> GDQLTHVVEEVKTYDLVWRSIKNLWEDVQRTFETPWCRVDVLLLQSDLANFLRRADELPRAVKQFEMYKSLFSQVNMLTSVNKILVELKDGALKPRHWNMIFRDIGKRQIQKNLLDKLEFSLKDVMVLNLTLNEILLTKIIERAQKEFVIEKSLNRIKKFWKEAQYEVIEHSSGLKLVREWDVLEQACKEDLEELVSMKASNYYKIFEQDCLDLESKLTKLSEIQVNWVEVQFYWLDLYGILGENLDIQNFLPLETSKFKSLTSEYKMITTRAFQLDTTIEVIHIPNFDTTLKLTIDSLKMIKSSLSTFLERQRRQFPRFYFLGNDDLLKIIGSGKHHDQVSKFMKKMFGSIESIIFFEDSITGVRSVEGEVLNLNEKIELKDSIQAQEWLNILDTEIKLSVFTQFRDCLGQLKDGTDIEVVVSKYIFQAILLSAQVMWTELVEKCLQTNEFSKYWKEVDMKIKGLLDKLNKSSDNVKKKIEALLVEYLHFNNVIGQLKNCSTKEEARLLWAKVQKFYQKNDTLDDLNSVFISQSGYLLQYKFEYIGIPERLIYTPLLLVGFATLTDSLHQKYGGCFFGPAGTGKTETVKAFGQNLGRVVVVFNCDDSFDYQVLSRLLVGITQIGAWGCFDEFNRLDEKVLSAVSANIQQIQNGLQVGKSHITLLEEETPLSPHTAVFITLNPGYNGRSELPENLKKSFREFSMKSPQSGTIAEMILQIMGFEDSKSLASKIVHFLELLSSKCSSMNHYHFGLRTLKGVLRNCSPLVSEFGEGEKTVVESLKRVILPSLGDTDELVFKDELSKIFDSAGTPLNSKAIVQCLKDAGQRSGFSMSEEFLKKCMQFYYMQKTQQALILVGKAGCGKTATWKTVIDAMAIFDGHANVVYVIDTKVLTKESLYGSMLKATLEWRDGLFTSILRRVNDDITGTFKNSRIWVVFDSDLDPEYVEAMNSVLDDNKILTLPNGERLPIPPNFRILFETDNLDHTTPATITRCGLLWFSTDVCSISSKIDHLLNKSYEALDNKLSMFELDKLKDLISDSFDMASLTNIFTCSNDLVHILGVRTFNKLETAVQLAVHLISSYRQWFQNLDDKSLKDVITLLIKRSLLYALAGDSTGESQRAFIQTINTYFGHDSQELSDYSTIVIANDKLSFSSFCSEIPSVSLEAHEVMRPDIVIPTIDTIKHEKIFYDLLNSKRGIILCGPPGSGKTMIMNNALRNSSLYDVVGINFSKDTTTEHILSALHRHTNYVTTSKGLTLLPKSDIKNLVLFCDEINLPKLDKYGSQNVVLFLRQLMEKQGFWKTPENKWVTIERIHIVGACNPPTDPGRIPMSERFTRHAAILYLGYPSGKSLSQIYEIYYKAIFKLVPEFRSYTEPFARASVHLYNECKARYSTGLQSHYLFSPRELTRLVRGVYTAINTGPRQTLRSLIRLWAYEAWRIFADRLVGVKEKNSFEQLLYETVDKYLPNQDLGNISSTSLLFSGLLSLDFKEVNKTDLVNFIEERFKTFCDEELEVPMVIHESMVDHILRIDRALKQVQGHMMLIGASRTGKTILTRFVAWLNGLKIVQPKIHRHSNLSDFDMILKKAISDCSLKESRTCLIIDESNILETAFLERMNTLLANADIPDLFQGEEYDKLLNNLRNKTRSLGLLLDTEQELYDWFVGEIAKNLHVVFTICDPTNNKSSAMISSPALFNRCIINWMGDWDTKTMSQVANNMVDVVPMEFTDFIVPEVNKELVFTEPIQTIRDAVVNILIHFDRNFYQKMKVGVNPRSPGYFIDGLRALVKLVTAKYQDLQENQRFVNVGLEKLNESVLKVNELNKTLSKKSTELTEKEKEARSTLDKMLMEQNESERKQEATEEIKKILKVQEEDIRKRKEVVMKSIQDIEPTILEAQRGVKNIKKQQLTEIRSMVNPPSGVKIVMEAVCAILGYQFSNWRDIQQFIRKDDFIHNIVHYDTTLHMKPQIRKYMEEEFLSDPNFTYETINRASKACGPLYQWVNAQINFSKVLENVDPLRQEMKRIEFESLKTKANLLAAEEMTQDLEASIEVSKQKYSLLIRDVEAIKTEMSNVQANLDRSISLVKSLTFEKERWLNTTKQFSKTSQELIGNCIISSIYETYFGHLNERERGDMLVILKRLLGKFAVKYDVNYRFIDYLVTLDEKMKWLECGLDKNDYFLENMSIVMNSQDAVPFLLDPSSHMITVISNYYGNKTVLLSFLEEGFVKRLENAVRFGSVVIIQDGEFFDPIISRLISREFNHAGNRVTVEIGDHEVDVSGDFKLFIHSCDPSGDIPIFLRSRVRLVHFVTNKESIETRIFDITLTEENAEMQRKREDLIKLNTEYRLKLKNLEKRLLEELNNSQGNMLENDELMVTLNNLKKEAMNIEKKLSESEEFFPQFDNLVEEYSIIGKHSVKIFSMLEKFGQFHWFYGISIGQFLSCFKRVFIKKSRETRAARTRVDEILWLLYQEVYCQFSTALDKKFKMIMAMTMFCLYKFDIESEQYKEAVLTMIGVLSESSDGVPKLTVDTNDDLRYLWDYVTTKSYISALNWFKNEFFVDEWNIADVVANSENNYFTMASERDVDGTFKLIELAKASKESLKIIPLGSIENLNYAQEEISKSKIEGGWILLQNIQMSLSWVKTYLHKHVEETKAAEEHEKFKMFMTCHLTGDKLPAPLLQRTDRVVYEDIPGILDTVKDLWGSQFFTGKISGVWSVYCTFLLSWFHALITARTRLVPHGFSKKYYFNDCDFQFASVYLENVLATNSTNNIPWAQVRDHIATIVYGGKIDEEKDLEVVAKLCAHVFCGSDNLQIVPGVRIPQPLLQQSEEEERARLTAILSNTIEPADSLSSWLQLPRESILDYERLQAKEVASSTEQLLQEM;>GMTNWQQQLPLTDTQKNELDKSVLRYLNWNYKQTVRHEHAQDYESVRHAIVTLSGFLLQESVDRQEFISNNDTSNESMVDIDELLLPKKWNSIVRLQKKIIELEQNTETLVSQIKDLNTQVSELAQFKPTTSNGTSAHNVLKWIPRNLPSCLINVESSVTSVKLHPNLPIVFVATDHGKLYAFDLFNYTIPLASLQSHTKAITSMDVLFTNYTNSSKKNYLVIVTASKDLQIHVFKWVSEECKFQQIRSLLGHEHIVSAVKIWQKNNDVHIASCSRDQTVKIWDFHNGWSLKTFQPHSQWVRSIDVLGDYIISGSHDTTLRLTHWPSGNGLSVGTGHEFPIEKVKFIHFIEDSPEIRFRTPSTDRYKNWGMQYCVSASRDRTIKIWEIPLPTLMAHRAPIPNPTDSNFRCVLTLKGHLSWVRDISIRGQYLFSCADDKSVRCWDLNTGQCLHVWEKLHTGFVNCLDLDVDFDSNVTPRQMMVTGGLDCKSNVFMR[2x]

Cytoplasmic dynein-1 (dynein) is a highly conserved molecular motor that moves toward the microtubule minus end, transporting various cargoes including RNAs, membrane vesicles, and viruses, and plays a crucial role in cell division. Dynein belongs to the ATPase associated with various cellular activities (AAA+) family of proteins. Its heavy chain features a motor domain composed of six AAA+ modules, a long stalk, a microtubule-binding domain (MTBD) located at the end of the stalk, a buttress region that makes additional connections between the AAA5 module and the stalk, and a long tail that interacts with dynactin and an activating adapter. Lis1 is a dimer (~90 kDa) with an amino-terminal dimerization domain and carboxy-terminal β-propellers that bind to the dynein motor domain24,25. Our data support a model in which Lis1 relieves dynein autoinhibition by increasing its basal ATP hydrolysis rate and promoting conformations compatible with complex assembly and motility.

We also prepared grids with samples that were pre-incubated with Lis1 before ATP addition. Because some of our maps showed partial density for the Lis1 β-propellers, we performed 3D classifications without alignment in Relion to further resolve this compositional heterogeneity. This analysis distinguished states with no, one, or two Lis1 β-propellers bound to dynein. The nucleotide occupancies in these new maps correspond to the nucleotides observed in pre-3D classification maps. In addition, the interaction sites between Lis1 and dynein in our maps are those previously characterized and are largely the same in the bent and intermediate dynein states. We also saw clear density for the second Lis1 β-propeller in the intermediate state dynein, even though the nucleotide densities in this state are consistent with the ones in the straight linker dynein. Comparison of this state (I6, 3.4-Å resolution) with our straight linker dynein (I3, 4-Å resolution) bound to one Lis1 β-propeller showed that the sitering interactions are conserved while sitestalk is shifted away from Lis1 as dynein goes from the intermediate to the straight linker state (~15 Å), making it inaccessible for binding by the second Lis1 β-propeller. Binding of Lis1 at the second site is unlikely to happen without Lis1 bound at sitering. We next investigated the AAA3 and AAA4 contact area and showed that Lis1 binding loosens the AAA3 and AAA4 interface, potentially favoring ADP release from the AAA3 binding pocket. Notably, binding of the second Lis1 β-propeller further loosens the interface, as illustrated by comparing the population distributions of interm-2× Lis1 versus interm-1× Lis1 systems.4-(3,5-DIMETHYLPHENOXY)-5-(FURAN-2-YLMETHYLSULFANYLMETHYL)-3-IODO-6-METHYLPYRIDIN-2(1H)-ONE | C20 H20 I N O3 S | 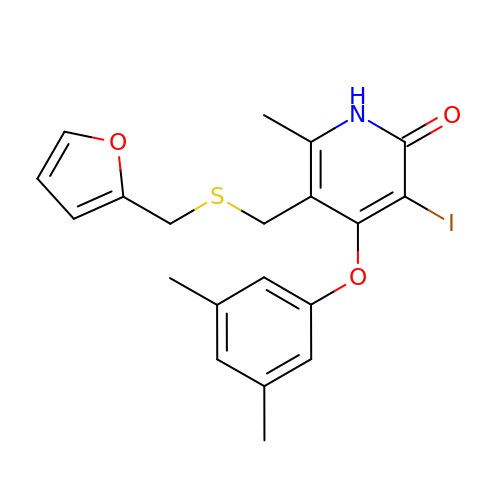YZLKVEDFWLGNQP-UHFFFAOYSA-N>[2x]MSSSHHHHHHMPTKKQKSKSKLKPFFALVRRTNPSYGKLAFALALSVVTTLVSLLIPLLTKQLVDGFSMSNLSGTQIGLIALVFFVQAGLSAYATYALNYNGQKIISGLRELLWKKLIKLPVSYFDTNASGETVSRVTNDTMVVKELITTHISGFITGIISVIGSLTILFIMNWKLTL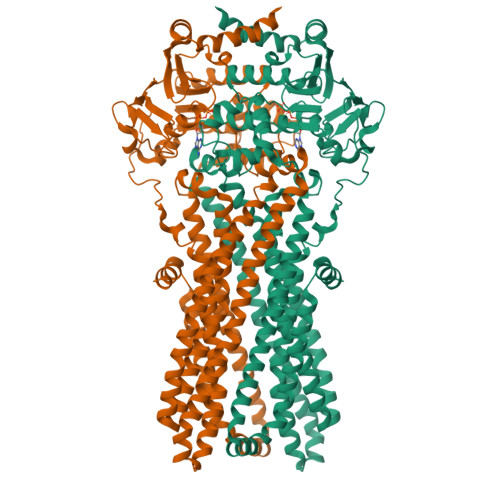LVLVVVPLAALILVPIGRKMFSISRETQDETARFTGLLNQILPEIRLVKASNAEDVEYGRGKMGISSLFKLGVREAKVQSLVGPLISLVLMAALVAVIGYGGMQVSSGELTAGALVAFILYLFQIIMPMGQITTFFTQLQKSIGATERMIEILAEEEEDTVTGKQIENAHLPIQLDRVSFGYKPDQLILKEVSAVIEAGKVTAIVGPSGGGKTTLFKLLERFYSPTAGTIRLGDEPVDTYSLESWREHIGYVSQESPLMSGTIRENICYGLERDVTDAEIEKAAEMAYALNFIKELPNQFDTEVGERGIMLSGGQRQRIAIARALLRNPSILMLDAATSSLDSQSEKSVQQALEVLMEGRTTIVIAHRLSTVVDADQLLFVEKGEITGRGTHHELMASHGLYRDFAEQQLKMNADLEN> AFGQDGNNWMEIDDLAKGLPDDLFDFILFDACYMASVECTYELRNKAEYILASPTETMADGWPYEEMMPQLFATDLQLEKVGETFYNHYLNNTYPYATVSLTKTSELDNLKSAIHDILADKTESDIYSLDPKNMQRLEYLYRSPGMLYDFN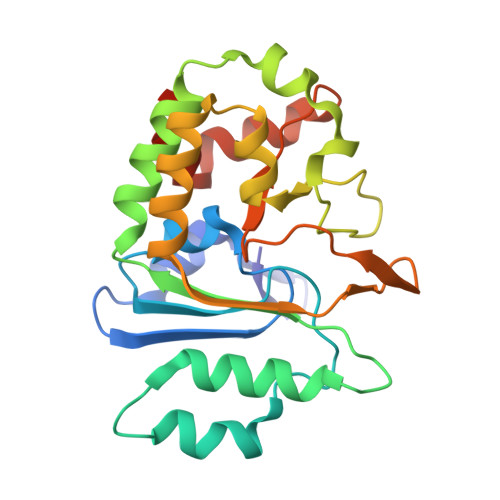DYIKQLATAEQYDRFISCLDKAVVYKAHTPKSYYAAIGNALPIKSYCGLTIFVPQESLPKMLEWYKQRVGWYKAVYELEHHHHHH> DNPPNEIYATAQQKLQDGNWRQAITQLEALDNRYPFGPYSQQVQLDLIYAYYKNADLPLAQAAIDRFIRLNPTHPNIDYVMYM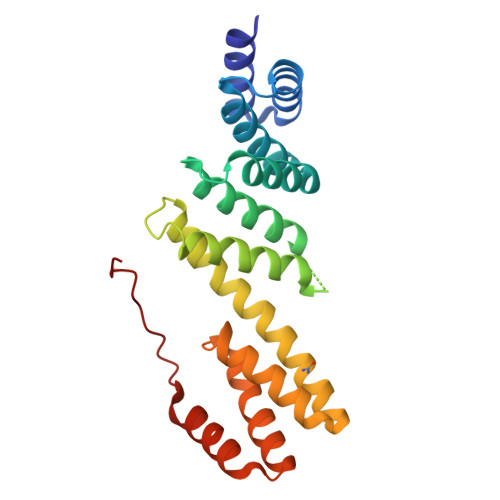RGLTNMALDDSALQGFFGVDRSDRDPQQARAAFSDFSKLVRGYPNSQYTTDATKRLVFLKDRLAKYEYSVAEYYTERGAWVAVVNRVEGMLRDYPDTQATRDALPLMENAYRQMQMNAQAEKVAKIIAANSSNTLEHHHHHH>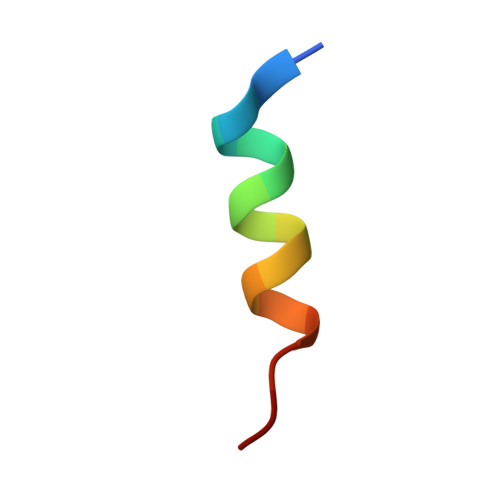 SEDDLLQECISSAMPK(1R,5S)-N-cyclopropyl-7-{4-[2-(2,6-dichloro-4-methylphenoxy)ethoxy]phenyl}-N-(2,3-dimethylbenzyl)-3,9-diazabicyclo[3.3.1]non-6-ene-6-carboxamide 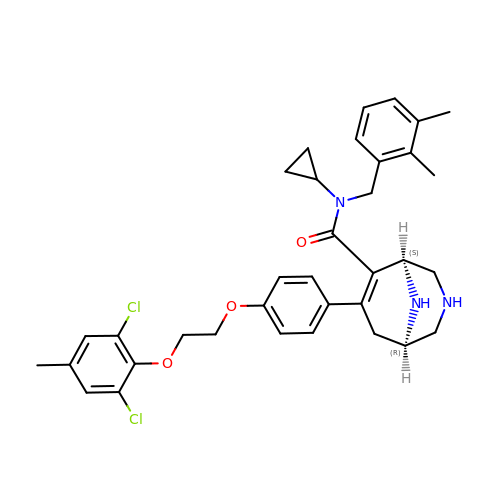| C35 H39 Cl2 N3 O3 | VKBBVOVNGWGZCA-HVIPQOSHSA-N Poxviruses are among the largest double-stranded DNA viruses, with members such as variola virus, monkeypox virus and the vaccination strain vaccinia virus (VACV). The core is one of the uniting factors in all the infectious poxvirus forms and fulfills one of the key roles in the virus lifecycle, that is the protected transfer of the viral genome and required accessory proteins to a newly infected cell. Room-temperature and cryo-electron microscopy (cryo-EM) analysis of VACV has revealed the presence of a regular, but discontinuous, palisade layer formed of spike-like assemblies on the outside of a continuous viral inner core wall. Here we show, using a multi-modal cryo-electron microscopy (cryo-EM) approach in combination with AlphaFold molecular modeling, that trimers formed by the cleavage product of VACV protein A10 are the key component of the palisade layer.

Our analysis revealed that hydrophobic interactions dominate within the 2,104-Å2 buried surface area per protomer pair. There are also several conserved inter-chain salt bridges tethering central alpha helices together within the trimer. Remarkably, each pair of protomers assembles a core heterodimeric three-stranded beta-sheet (residues 85–110), formed by two strands from one monomer and one strand from the neighboring monomer. A hydrogen bond network on the outward surface of the beta-sheet further reinforces this interaction, while the opposite side of the beta-sheet packs tightly with underlying hydrophobic side chains. When analyzing our A10 model, we found two highly conserved cysteine residues (C31 and C569) in close proximity to each other, which conceivably could clamp the N-terminal and C-terminal domains of A10 monomer together, stabilizing its conformation. The model of our trimer fits into our STA density map with high agreement, leaving no major area of density within the palisade layer unoccupied. This strongly suggests that the A10 trimer is the main constituent of the palisade layer. However, our fit into the STA map also revealed that the lateral interactions across trimers within the palisade layer are not extensive, given the wide spacing between them. Interestingly, the bottom of the A10 trimer facing the inner core wall is strongly positively charged.

>MMPIKSIVTLDQLEDSEYLFRIVSTVLPHLCLDYKVCDQLKTTFVHPFDILLNNSLGSVTKQDELQAAISKLGINYLIDTTSRELKLFNVTLNAGNIDIINTPINISSETNPIINTHSFYDLPPFTQHLLNIRLTDTEYRARFIGGYIKPDGSDSMDVLAEKKYPDLNFDNTYLFNILYKDVINAPIKEFKAKIVNGVLSRQDFDNLIGVRQYITIQDRPRFDDAYNIADAARHYGVNLNTLPLPNVDLTTMPTYKHLIMFEQYFIYTYDRVDIYYNGNKMLFDDEIINFTISMRYQSLIPRLVDFFPDIPVNNNIVLHTRDPQNAAVNVTVALPNVQFVDINRNNKFFINFFNLLAKEQRSTAIKVTKSMFWDGMDYEEYKSKNLQDMMFINSTCYVFGLYNHNNTTYCSILSDIISAEKTPIRVCLLPRVVGGKTVTNLISETLKSISSMTIREFPRKDKSIMHIGLSETGFMRFFQLLRLMADKPHETAIKEVVMAYVGIKLGDKGSPYYIRKESYQDFIYLLFASMGFKVTTRRSIMGSNNISIISIRPRVTKQYIVATLMKTSCSKNEAEKLITSAFDLLNFMVSVSDFRDYQS[3x]> GDRVADVIESSIGDSVSRALTRALPAPT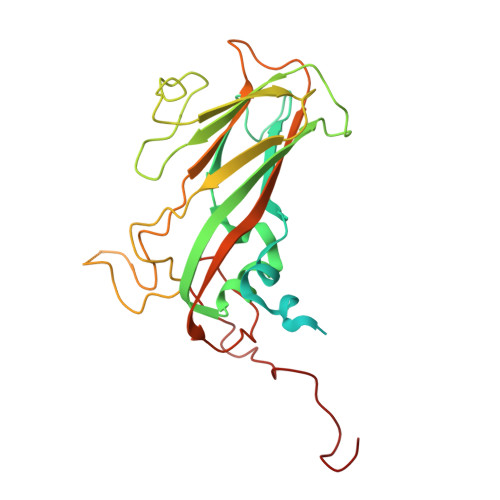GQNTQVSSHRLDTGKVPALQAAEIGASSNASDESMIETRCVLNSHSTAETTLDSFFSRAGLVGEIDLPLEGTTNPNGYANWDIDITGYAQMRRKVELFTYMRFDAEFTFVACTPTGGVVPQLLQYMFVPPGAPKPDSRESLAWQTATNPSVFVKLSDPPAQVSVPFMSPASAYQWFYDGYPTFGEHKQEKDLEYGACPNNMMGTFSVRTVGTSKSKYPLVVRIYMRMKHVRAWIPRPMRNQNYLFKANPNYAGNSIKPTGASRTAITTL>[4x]MEAGITGTWYNQLG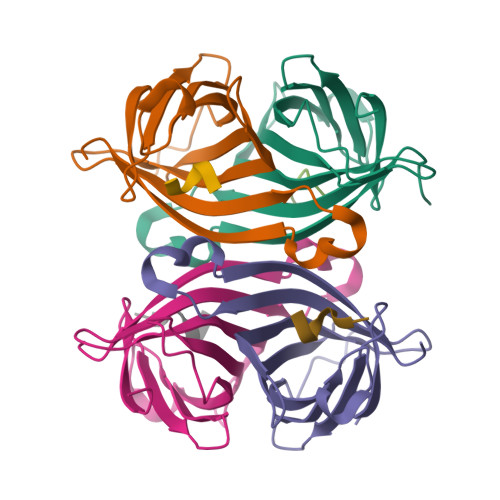STFIVTAGADGALTGTYIGARGNAESRYVLTGRYDSAPATDGSGTALGWTVAWKNNYRNAHSATTWSGQYVGGAEARINTQWLLTSGTTEANAWKSTLVGHDTFTKVKPSAAS;>[4x]NWSHPQFEK>SNAMK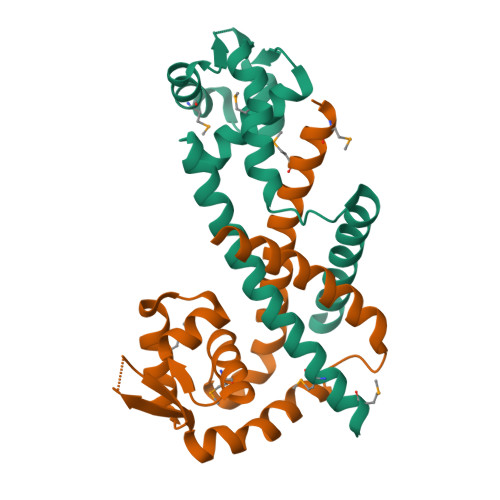QEQMRLANQLCFSAYNVSRLFAQFYEKKLKQFGITYSQYLVMLTLWEENPQTLNSIGRHLDLSSNTLTPMLKRLEQSGWVKRERQQSDKRQLIITLTDNGQQQQEAVFEAISSCLPQEFDTTEYDETKYVFEELEQTLKHLIEK[4x]>MQPVRFGSPWIMAIGLVLLLLAFVSAGKSRQRSPANCPTIKLKRQWGGKPSLGLHYQVRPIRYVVIHHTVTGECSGLLKCAEILQNMQAYHQNELDFNDISYNFLIGNDGIVYEGTGWGLRGAHTYGYNAIGTGIAFIGNFVDKLPSDAALQAAKDLLACGVQQGELSEDYALIAGSQVISTQSPGLTLYNEIQE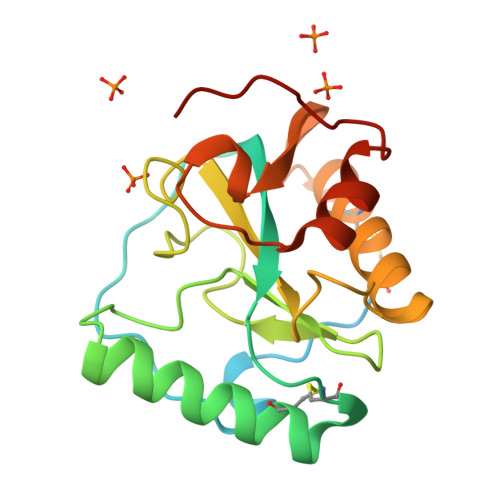WPHWLSNPHHHHHH[2x]> GENSDNLTHCRLFEFRLCLLECMSLTLDHCYARCTTVITQIHGSDTNRFDCTIFKTCYYRCYVLGKTEDHCWKGTATSVTGDVGDLEFC

The Mu8.1 conotoxin from Conus mucronatus is the founding member of the newly identified saposin-like conotoxin class of conotoxins and has been shown to target Cav2.3, a voltage-gated calcium channel. Two recently published crystal structures of C. mucronatus Mu8.1 revealed an all-helical molecule forming a homodimer, with a common dimer interface observed in two different crystal conditions. Each protomer in the dimer comprises five disulfide bonds connecting the four α-helices and shows structural similarity to saposin-like proteins as well as con-ikot-ikot from C. striatus. Five disulfide bonds contribute to the overall rigidity of the toxin by forming both interdomain and intradomain connections, referred to by the roman numerals I–V. The first domain is stabilized by two disulfide bonds formed by Cys18–Cys34 (I) and Cys22–Cys30 (II), both connecting α1 and α2.

Here, we present a high-resolution crystal structure of Mu8.1 obtained from a new crystal condition in the high-symmetry space group I4222 at 1.67 Å resolution. The structure reveals a dimer interface equivalent to that previously observed in Mu8.1; however, in the present crystal structure it is formed between two symmetry-related molecules. The high-resolution structure of Mu8.1 obtained in this work allowed us to identify a tightly coordinated hydrogen-bond network around Lys55. The network of water molecules revealed at 1.67 Å resolution surrounds a potential functional residue, Lys55, and may contribute to the unusually low pK a value (8.16) predicted for Lys55 by PROPKA. The relatively low side-chain pK a could imply that Lys55 is uncharged in the dimer, thus rationalizing how it can be accommodated at the hydrophobic dimer interface. Overall, we propose that the combination of this side-chain stacking and the observed hydrogen-bonding network creates a hydrophobic microenvironment surrounding Lys55 that results in a lowering of the pK a of its ɛ-amino group.>[2x]YVEIIEQPKQRGMRFRYKCEGRSAGSIPGERSTDTTKTHPTIKINGYTGPGTVRISLVTKDPPHRPHPHELVGKDCRDGFYEAELCPDRCIHSFQNLGIQCVKKRDLEQAISQRIQTNNNPFQVPIEEQRGDYDLNAVRLCFQVTVRDPSGRPLRLPPVLPHPIF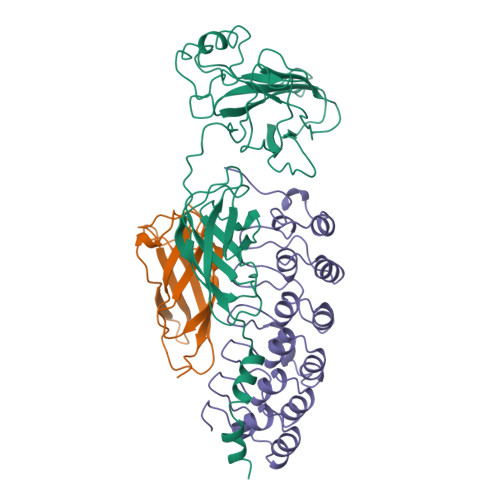DNRAPNTAELKICRVNRNSGSCLGGDEIFLLCDKVQKEDIEVYFTGPGWEARGSFSQADVHRQVAIVFRTPPYADPSLQAPVRVSMQLRRPSDRELSEPMEFQYLPDTDDRHRIEEKRKRTYETFKSIMKKSPFSG;>SNLKIVRMDRTAGCVTGGEEIYLLCDKVQKDDIQIRFYEEEENGGVWEGFGDFSPTDVHRQFAIVFKTPKYKDINITKPASVFVQLRRKSDLETSEPKPFLYYPEIK[2x];>LTEDGDSFLHLAIIHEEKALTMEVIRQVKGDLAFLNFQNNLQQTPLHLAVITNQPEIAEALLGAGCDPELRDFRGNTPLHLACEQGCLASVGVLTQSCTTPHLHSILKATNYNGHTCLHLASIHGYLGIVELLVSLGADVNAQEPCNGRTALHLAVDLQNPDLVSLLLKCGADVNRVTYQGYSPYQLTWGRPSTRIQQQLGQLTLENLQMLPE[2x]>AIDEI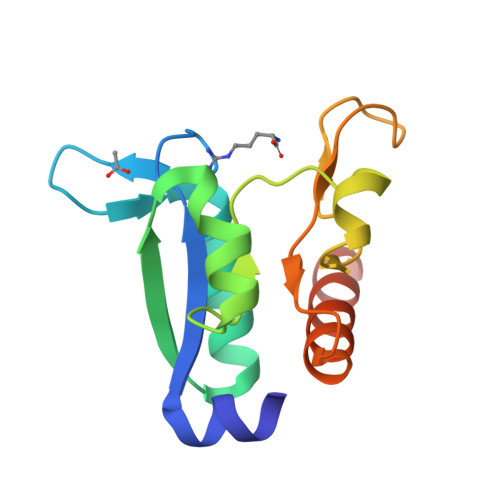KSRGYLLVGLSADFPPFEFVDENGNIVGFDVDLAKEIARRLGVELKIVDMTWDGLIPSLLTKKIDVIISGMTITEERKKVVAFSDPYFDAGGGGSGEQYGIAVRKEDTDLLEFINSVLRELKKLEHHHHHH[2x]>MNNMNVIIADDHPIVLFGIRKSLEQIEWVNVVG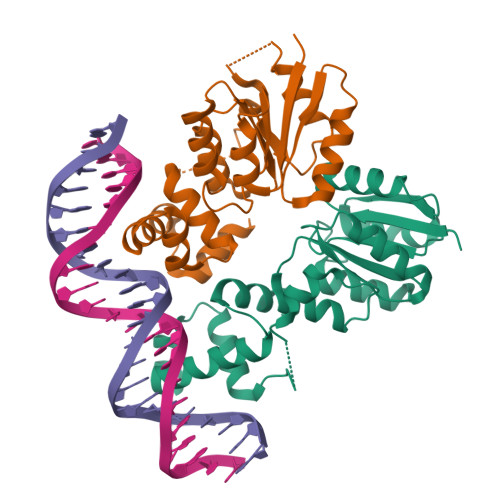EFEDSTALINNLPKLDAHVLITDLSMPGDKYGDGITLIKYIKRHFPSLSIIVLTMNNNPAILSAVLDLDIEGIVLKQGAPTDLPKALAALQKGKKFTPESVSRLLEKISAGGYGDKRLSPKESEVLRLFAEGFLVTEIAKKLNRSIKTISSQKKSAMMKLGVENDIALLNYLSSVTLSPADKD[2x]~{N}-[3-[1-[[4-(5-methyl-6-oxidanylidene-3-phenyl-1~{H}-pyrazin-2-yl)phenyl]methyl]piperidin-4-yl]-2-oxidanylidene-1~{H}-benzimidazol-5-yl]propanamide 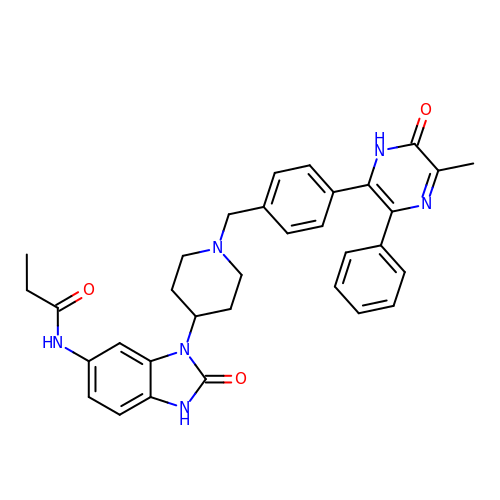| C33 H34 N6 O3 | HCHZPUXPCDNSSQ-UHFFFAOYSA-N>TKVKRDISAFQKVIQDISLAVNKFNVDIERYVGGDASHLLADGNVLIKATLDGVQSLQNEPPLSSMEALALVGPVQDLSNQILLAIQNLIDKKEPLVQAGFGGKVENNLRQQEEAAQKLSELVSTKVPHELADISRQLSDGIAAGIKKGID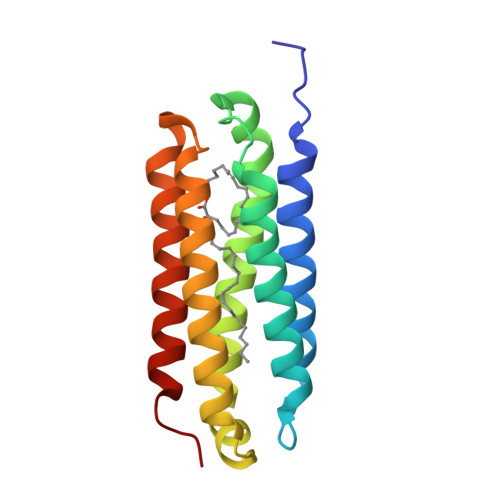AFAGTGPA[4x]>[2x]MELPNIMHPVAKLSTALAAALMLSGCMPGEIRPTIGQQMETGDQRFGDLVFRQLAPNVWQHTSYLDMPGFGAVASNGLIVRDGGRVLVVDTAWTDDQTAQILNWIKQEINLPVALAVVTHAHQDKMGGMDALHAAGIATYANALSNQLAPQEGMVAAQHSLTFAANGWVEPATAPNFGPLKVFYPGPGHTSDNITVGIDGTDIAFGGCLIKDSKAKSLGN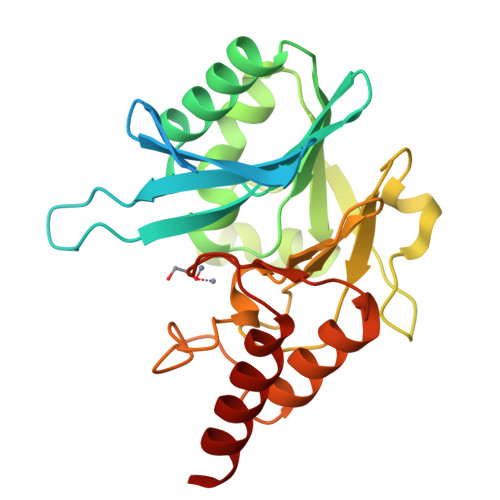LGDADTEHYAASARAFGAAFPKASMIVMSHSAPDSRAAITHTARMADKLRLV> MAPEAQVSVQPNFQQDKFLGRWFSAGLASNSSWLREKKAALSMCKSVVAPATDGG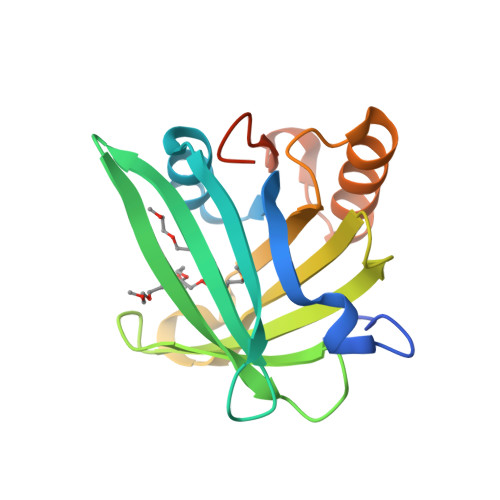LNLTSTFLRKNQCETRTMLLQPAGSLGSYSYRSPHWGSTYSVSVVETDYDQYALLYSQGSKGPGEDFRMATLYSRTQTPRAELKEKFTAFCKAQGFTEDTIVFLPQTDKCMTEQAHHHHHH> GQTADWKSIGLYILSFALPIILKALYMLSTRGRQTI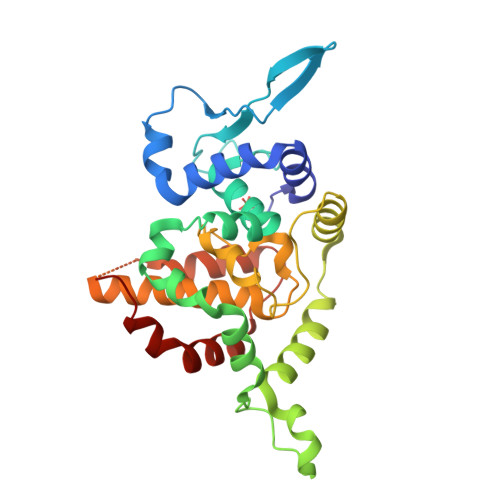KENKGTRIRFKDDSSYEEVNGIRKPRHLYVSMPTAQSTMKADEITPGRFRTIACGLFPAQVKARNIISPVMGVIGFSFFVKDWMERIDDFLAARCPFLPEQKDPRDAALATNRAYFITRQLQVDESKVSDIEDLIADARAESATIFADIATPHSVWVFACAPDRCPPTALYVAGMPELGAFFAILQDMRNTIMASKSVGTSEEKLKKKSAFYQSYLRRTQSMGIQLDQKIIILYMSHWGREAVNHFHL>MKEHRHMTEKSPHSAFGDGAKAYDVPAFGLQIHTVEHGSGAPIVFLHGNPTSSYLWRHIFRRLHGHGRLLAVDLIGYGQSSKPDIEYTLENQQRYVDAWFDALDLRNVTLVLQDYGAAFGLNWASRNPDRVRAVAFFEPVLRNIDSVDLSPEFVTRRAKLRQPGEGEIFVQQENRFLTELFPWFFLTPLAPEDLRQ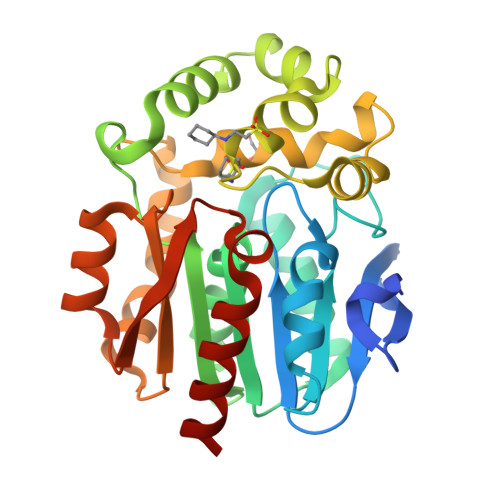YQTPFPTPHSRKAILAGPRNLPVDGEPASTVAFLEQAVNWLNTSDTPKLLLTFKPGFLLTDAILKWSQVTIRNLEIEAAGAGIHFVQEEQPETIARLLDAWLTRIAGN[2x]> MSNTVTLRADGRLFTGWTSVSVTRSIESVAGYFELGVNVPPGTDLSGLAPGKKFTLEIGGQIVCTGYIDSRRRQMTADSMKITVAGRDKTADLIDCAAVYSGGQWKNRTLEQIARDLCAPYGVTVRWELSDKESS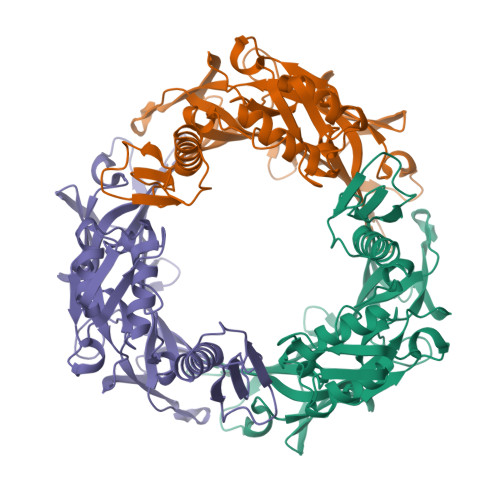AAFPGFTLDHSETVYEALVRASRARGVLMTSNAAGELVFSRAASTATDELVLGENLLTLDFEEDFRDRFSEYTVKGYARANGAEGDDIDAKSIVSRKGTATDSDVTRYRPMIIIADSKITAKDAQARALREQRRRLAKSITFEAEIDGWTRKDGQLWMPNLLVTIDASKYAIKTTELLVSKVTLILNDQDGLKTRVSLAPREGFLVPVESDRKNRKGGDSNGGIDALVEDYYRRHPEKTPPWKE4-[[[4-imidazol-1-yl-3-[1-[(4-methoxyphenyl)methyl]-3-methyl-pyrazol-4-yl]phenyl]methylamino]methyl]-~{N}-methyl-benzamide | 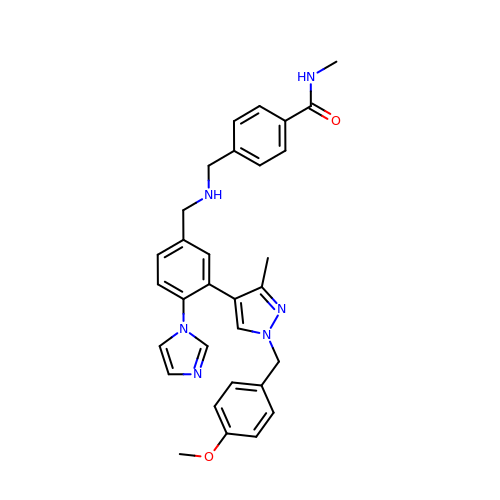C31 H32 N6 O2 | BOWNAJGILQQXOM-UHFFFAOYSA-N> GAMAGMNIKDRTSEFQQSVLSYKKRNKNFREQQRERLQEKESE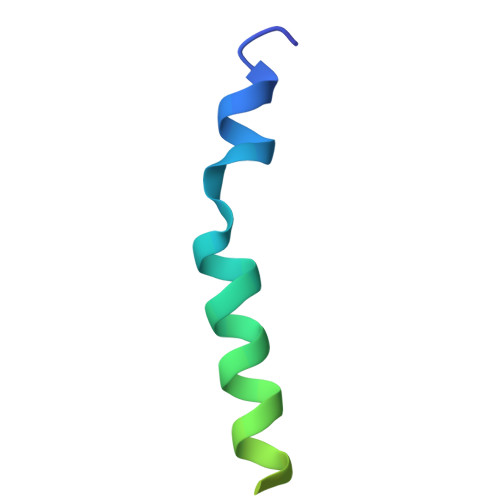NFANNTT Glutamine synthetases (GS) catalyze the ATP-dependent ammonium assimilation, the initial step of nitrogen acquisition that must be under tight control to fit cellular needs. The dodecamer is organized as two stacked hexameric rings, and each polypeptide is organized into two parts, a shorter N-terminal domain (β-Grasp fold) and the remaining C-terminal domain. The active sites are located at the interface of the N- and C- terminal domains of the adjacent subunit in the hexameric ring. Two loops in the active center are critical for catalysis: the Glu-flap, involved in shielding the active site during catalysis and deprotonating the intermediate product, and the Asp-50’ loop, which binds and deprotonates ammonium.

The enzyme from M. shengliensis was crystallized in the absence of ligands, and two different crystalline forms, referred to as MsGS-apo 1 and MsGS-apo 2, were analyzed. MtGS-apo-TbXo4 was selected as a template for molecular replacement, and the structures were refined to 2.64 Å and 3.09 Å, respectively. As MtGS, the homolog from M. shengliensis has a dodecameric organization with the N-ter (1-106) and C-ter (107-442) domains forming the protomeric unit.

>[2x]MGSKEDEIFRIVEEKNVRFVRLQFVDVQGIPKNVAIPVGQLEKALGPGIHFDGSSIEGFVRIEESDMVLRPDPDTFRVLPWSGNEGTAEARLICDIELPDGKPFMGCPRQVLKKNMEEAAKLGYVMNTGPEMEFFLFKRQDGMPTNIPQDRGGYFDLAPIDLAEEIKREIVLVLEEMGFEVEAAHHEVAFGQHEIDFKYDNALATADNVITLKYVAKTLALQHGLHATFMPKPIFGVNGSGMHTNTSLFKDGKNAFYDPDAPDQISDTLRYFVGGVLKHIRAITAITNPLVNSYKRLVPGYEAPVYITWSGPNRSSLIRVPAPRGNSTRIEIRSPDPSCNPYLAFAAILAAGLDGVKNKIEPPERVEKNIYKLTEEEREKLGIGMLPGTLKEAIECFKEDELLVSALGEHVSQSIINVAMADWDSYRTQVHQWELDRYLQTY> QIRYPVPEESQEGTFVGNVAQDFLLDTESLSARRLQVAGEVNQRHFRVDLDSGALLIKNPIDREALCGLSASCIVPLEFVTEGPLEMYRAEVEIVDVNDHAPRFPRQQLDLEIGEAAPPGQRFPLEKAQDADVGSNSISSYRLSSNEHFALDVKKRSDGSLVPELLLEKPLDREKQSDYRLVLTAVDGGNPPRSGTAELRVSVLDVNDNAPAFQQSSYRISVLESAPAGMVLIQLNASDPDLGPSGNVTFSFSGHTPDRVRNLFSLHPTTGKLTLQGPLDFESENYYEFDVRARDGGSPAMEQHCSLRVDLLDVNDNAPHITVTSELGTLPESAEPGTVVALISVQDPDSGSNGDVSLRIPDHLPFALKSAFRNQFSLVTAGPLDREARSSYDIMVTASDAGNPPLSTHRTIFLNISDVNDHHHHHHHH

Clustered protocadherins (cPcdhs) are a large family of cadherin-like proteins named for the clustered arrangement of their genes in vertebrate genomes. cPcdhs play roles in many facets of neural development, including circuit development, most notably neurite self-avoidance in vertebrates, and tiling. In mammalian nervous systems, cPcdh isoform expression is controlled by the unique organization of three tandem gene clusters, Pcdhα, Pcdhβ, and Pcdhγ, with each cluster containing multiple variable exons, which encode full cPcdh ectodomain regions with six extracellular cadherin (EC) domains, a single transmembrane region, and a short cytoplasmic extension. The last two variable exons in the Pcdhα gene cluster and the last three variable exons of the Pcdhγ gene cluster diverge in sequence from other cPcdh isoforms and are referred to as ‘C-type’ cPcdhs. Moreover, Garrett et al. discovered that neuronal survival and postnatal viability are controlled solely by γC4 suggesting a function that is unique to this isoform (although it presumably requires β and/or other γ carriers to reach the cell surface).

The biophysical properties of C-type cPcdhs pose a number of interesting questions: Despite their more divergent sequences compared with alternate cPcdhs, AUC data have confirmed that C-type cPcdhs αC2, γC3, and γC5 form trans dimers using their EC1–4 domains. However, γC41–4 behaved as a very weak dimer in AUC (KD >500 μM; Figure 2—source data 1), nevertheless full-length γC4 can mediate cell aggregation when delivered to the cell surface by coexpression with a ‘carrier’ cPcdh. However, there are no published crystal structures of C-type cPcdh trans dimers. We therefore sought to crystallize a mouse C-type cPcdh engaged in a trans interaction and obtained two distinct crystal forms of γC4EC1–4, one at 2.4 Å resolution (crystallized at pH 7.5) and the other with anisotropic diffraction at 4.6/3.9/3.5 Å resolution (Figure 3—source data 1) (crystallized at pH 6.0). Right, close-up view of the gap region in the crystal form two dimer with the side chains depicted as sticks. The intact crystal form 1 γC4 dimer is similar overall to those of the published intact alternate α, β, γA, and γB cPcdhs and the published δ2 nonclustered (nc) Pcdh trans dimers (root mean square deviation [RMSD] over aligned Cαs 2.4–4.5 Å; Figure 3—source data 2). The two most structurally similar molecules to γC4 over their trans-interacting domains are cPcdh γB2 and nonclustered Pcdh19. γB2 and Pcdh19 have trans dimer KDs of 21.8 and 0.48 μM, respectively, while that of γC4 is >500 μM. Comparison between the γB2 and γC4 dimer interfaces highlighted two buried charges in the γC4 trans interface, E78 and D290, which could potentially contribute to the low interaction affinity.> GEIQWVKPNKETGRLNINGPTRTKLEPSVFHDVFEGNKEPAVLHSKDPRLEVDFEQALFSKYVGNTLYEPDEYIKEAALHYANQLKQLDIDTSQMSMEEACYGTENLEAIDLHSTAGYPYSALGIKKRDILDSTTRDVSKMKFYMDKYGLDLPYSTYVKDELRSIDKIKKGKSRLIEASSLNDSVYLRMTFGHLYETFHA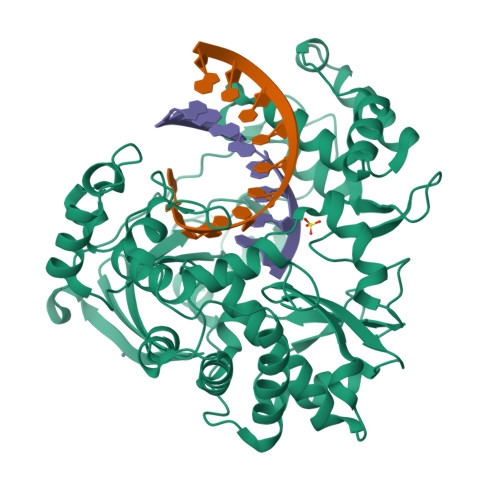NPGTVTGSAVGCNPDTFWSKLPILLPGSLFAFDYSGYDASLSPVWFRALELVLREIGYSEEAVSLVEGINHTHHVYRNKTYCVLGGMPSGMSGTSIFNSMINNIIIRALLIKTFKGIDLDELNMVAYGDDVLASYPFPIDCLELARTGKEYGLTMTPADKSPCFNEVNWDNATFLKRGFLPDEQFPFLIHPTMPMKEIHESIRWTKDARNTQDHVRSLCLLAWHNGKQEYEKFVSAIRSVPVGKALAIPNYENLRRNWLELFHHHHHH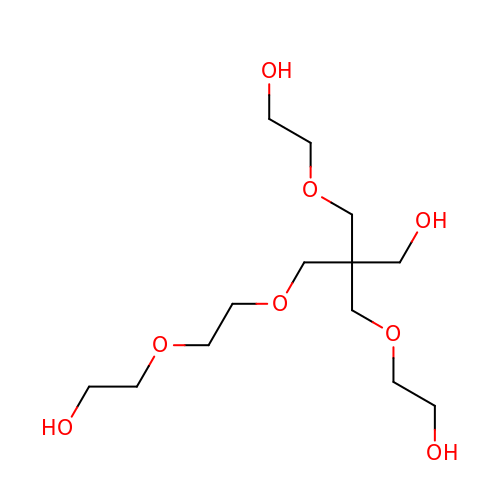3-(2-hydroxyethyloxy)-2-[2-(2-hydroxyethyloxy)ethoxymethyl]-2-(2-hydroxyethyloxymethyl)propan-1-ol | C13 H28 O8 | CLVWRDZKTFFQRY-UHFFFAOYSA-N> MKLKHLDKLLAHCHRRRYTAKSTIIYAGDRCETLFFIIKGSVTILIEDDDGREMIIGYLNSGDFFGELGLFEKEGSEQERSAWVRAKVECEVAEISYAKFRELSQQDSEILYTLGSQMADRLRKTTRKVGDLAFLDVTGRVARTLLD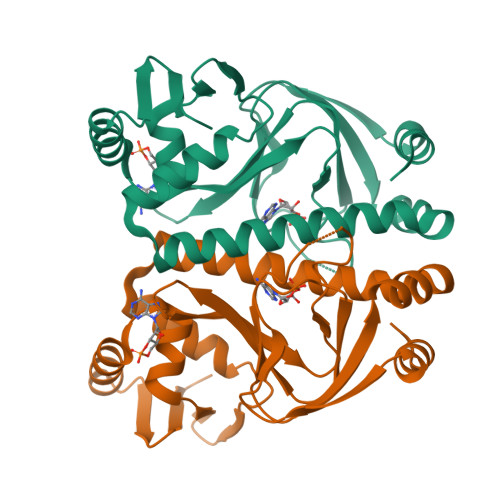LCQQPDAMTHPDGMQIKITRQEIGRIVGCSREMVGRVLKSLEEQGLVHVKGKTMVVFGTR> HHHHHHHHSQAGDTLNDVIQDPTRRNKLINDNNLLKGIIMGRDGPVPSS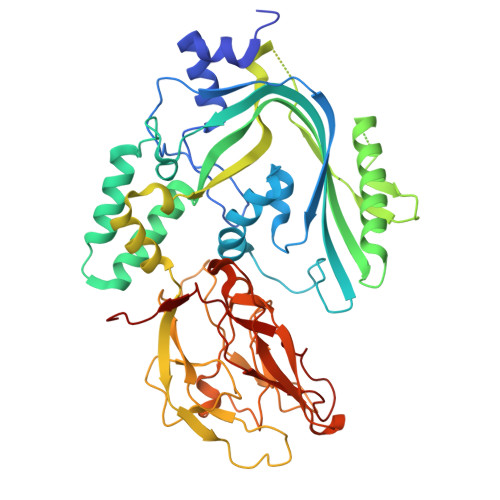RELIVRPDTLRAIINNRATIETTTMEAEFTETLMESNYNSASVKVSAPFITANSEYSESSSFKNTETEKSMYTSSRYLFPQGRIDFTTPDSGFDDVIKLSPQFTSGVQAALAKATGTEKREALQNLFQEYGHVFRTKVHIGGVLSAHTMETFSRSENETEVKQDVKAGLEGAVKGWGGGATAGHGNTQGTITTSQNRKLNVKYIVNVVDYTKIQNTEEWVASTNQSEHWRVIEVTEVTAVADLLPQPIRGQVKDLLKPLLGKWVDVEKVPGLESLPVSVYRPKGAIPAGWFWLGDTADASKALLVKPTLPARSGRNPALTSLHQGSGMTEQPFVDLPQYQYLSTYFGSFAHDTPPGSTLRGLRPDHVLPGRYEMHGDTISTAVYVTRPVDVPFPEDECFDLKSLVRVKLPGSGNPPKPRSALKKSMVLFDSGEK> G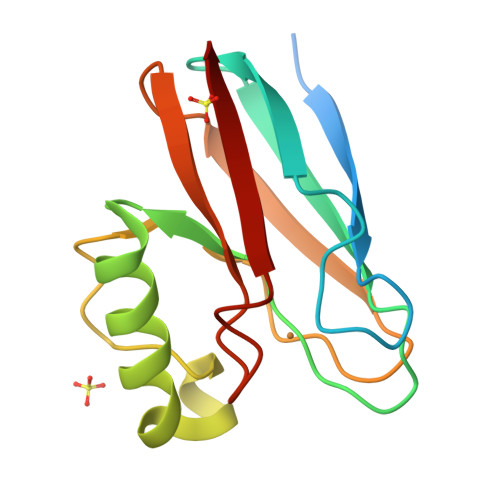GGGSSGGSTGGGSGSGPVTIEIGSKGEELAFDKTELTVSAGQTVTIRFKNNSAVQQHNWILVKGGEAEAANIANAGLSAGPAANYLPADKSNIIAESPLANGNETVEVTFTAPAAGTYLYICTVPGHYPLMQGKLVVN> MSLLERLNQDMKLYMKNREKDKLTVVRMVKASLQNEAIKLKKDSLTEDEELTVLSRELKQRKDSLQEFSNANRLDLVDKVQKE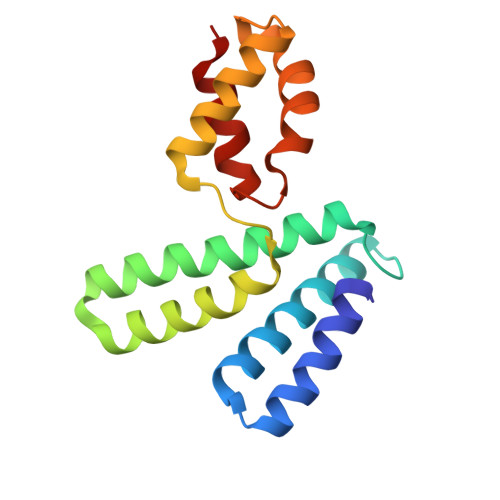LDILEVYLPEQLSEEELRTIVNETIAEVGASSKADMGKVMGAIMPKVKGKADGSLINKLVSSQLS>LTDLGGELSIKIKNEDLTFIAEKNSFSEEPFQDEIVSYNTKNKPLNFNYSLDKIIVDYNLQSKITLPNDRTTPVTKGIPYAPEYKSNAASTIEIHNIDDNTIYQYLYAQKSPTTLQRITMTNSVDDALINSTKIYSYFPSVISKVNQGAQGILFLQWVRDIIDDFTNESSQKTTIDKISDVSTIVPYIGPALNIVKQGYEGNFIGALETTGVVLLLEYIPEITLPVIAALSIAESSTQKEKIIKTIDNFLEKRYEKWIEVYKLVKAKWLGTVNTQFQKRSYQMYRSLEYQV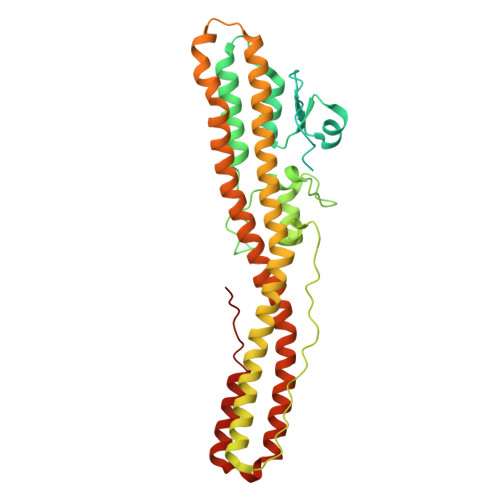DAIKKIIDYEYKIYSGPDKEQIADEINNLKNKLEEKANKAMININIFMRESSRSFLVNQMINEAKKQLLEFDTQSKNILMQYIKANSKFIGITELKKLESKINKVFSTPIPFSYS[2x]> MSEKKEARVVINDLLAEQYANAFKAKEEGRPVGWSTSVFPQELAEVFDLNVLYPENQAAGVAAKKGSLELCEIAESKGYSIDLCAYARTNFGLLENGGCEALDMPAPDFLLCCNNICNQVIKWYENISRELDIPLIMIDTTFNNEDEVTQSRIDYIKAQFEEAIKQLEIISGKKFDPKKFEEVMKISAENGRLWKYSMSLPADSSPSPMNGFDLFTYMAVIVCARGKKETTEAFKLLIEELEDNMKTGKSSFRGEEKYRIMMEGIPCWPYIG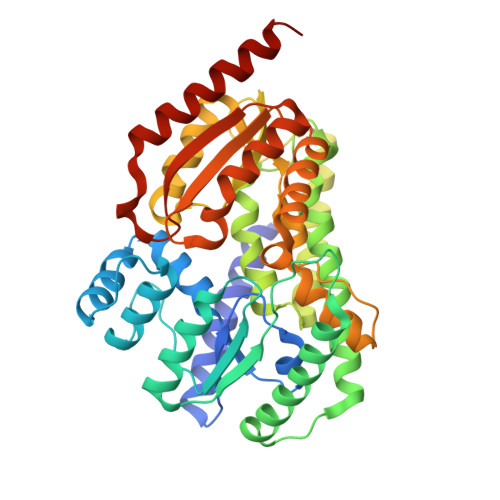YKMKTLAKFGVNMTGSVYPHAWALQYEVNDLDGMAVAYSTMFNNVNLDRMTKYRVDSLVEGKCDGAFYHMNRSCKLMSLIQYEMQRRAAEETGLPYAGFDGDQADPRAFTNAQFETRIQGLVEVMEERKKLNRGEI>MGQIFSRSASPIPRPPRGLAAHHWLNFLQAAYRLEPGPSSYDFHQLKKFLKIALETPARICPINYSLLASLLPKGYPGRVNEILHILIQTQAQIPSRPAPPPPSSPTHDPPDSDPQIPPPYVEPTAPQVLPVMHPHGAPPNHRPWQMKDLQAIKQEVSQAAPGSPQFMQTIRLAVQQFDPTAKDLQDLLQYLCSSLVASLHHQQLDSLISEAETRGITGYNPLAGPLRVQANNPQQQGLRREYQQLWLAAFAALPGSAKDPSWASILQGLEEPYHAFVERLNIALDNGLPEGTPKDPILRSLAYSNANKECQKLLQARGHTNSPLGDMLRACQTWTPKDKTKVLVVQPKKPPPNQPCFRCGKAGHWSRDCTQPRPPPGPCPLCQDPTHWKRDCPRLKPTIPEPEPEEDALLLDLPADIPHPKNSIGGEV[2x]

The retroviral structural protein Gag forms the immature protein shell of nascent virus particles4. All retroviral Gag proteins contain three canonical domains: matrix (MA), capsid (CA), consisting of independently folded N-terminal (CA-NTD) and C-terminal (CA-CTD) domains, and nucleocapsid (NC). During immature virus particle formation, these domains function in membrane binding, viral lattice self-assembly and viral genomic RNA (vgRNA) packaging, respectively. Our results show that HTLV-1 uses a distinct CA-NTD arrangement to form the immature Gag lattice and that, in contrast to other retroviral structures, the CA-NTD is the key determinant of immature HTLV-1 assembly.

To gain insight into the immature architecture of HTLV-1, we used cryo-ET to visualize mammalian cell-derived Gag-based VLPs. However, to account for the observed heterogeneity of HTLV-1 Gag VLP shapes, we applied local C2 symmetry during subtomogram averaging. The resulting maps had a CA-CTD layer that was resolved to a lower resolution than the CA-NTD layer, which we predict is because of heterogeneity caused by flexibility of the CA-CTD. Three-dimensional (3D) classification focused on the CA-CTD yielded a class in which all helices were resolved. Therefore, we used both domains as independent species in a multiparticle refinement using the software M34. This approach yielded 5.9-Å and 6.2-Å resolution maps of the CA-NTD and CA-CTD layers, respectively. Within the CA-CTD layer, the only intermolecular contact is a dimerization interface formed by helix 8. Unlike other retroviruses, where the CA-CTD forms interhexameric and intrahexameric contacts, the CA-CTD of HTLV-1 only forms interhexameric contacts. The positioning of the individual HTLV-1 CA-CTD dimers places them out of reach of the adjacent dimers around the hexameric CA ring, not enabling them to contribute to intrahexamerization interfaces forming a lattice. The positions of individual dimers are constrained only by the flexible linker between CA-NTD and CA-CTD.> MEDISEPPLHDFYCSRLLDLVFLLDGSSRLSEAEFEVLKAFVVDMMERLRISQKWVRVAVVEYHDGSHAYIGLKDRKRPSELRRIASQ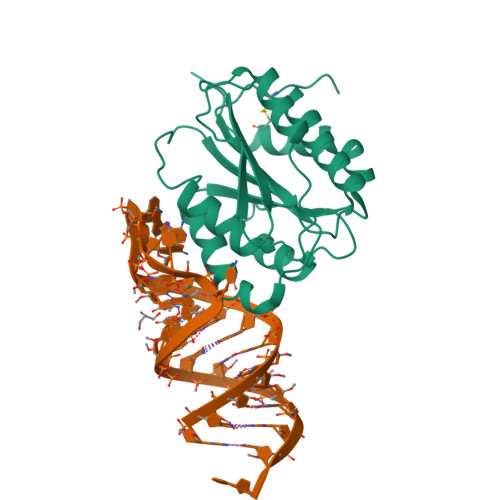VKYAGSQVASTSEVLKYTLFQIFSKIDRPEASRIALLLMASQEPQRMSRNFVRYVQGLKKKKVIVIPVGIGPHANLKQIRLIEKQAPENKAFVLSSVDELEQQRDEIVSYLCDLAPEAPPPT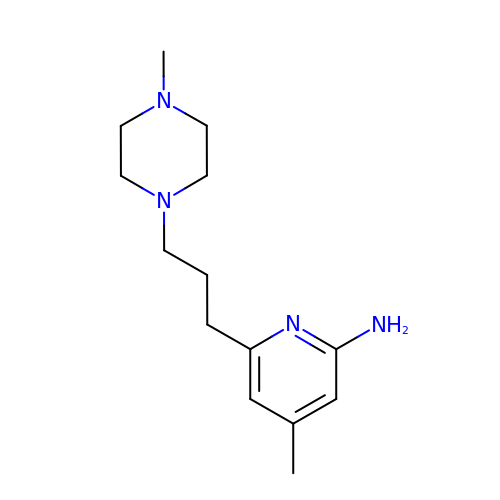4-methyl-6-[3-(4-methylpiperazin-1-yl)propyl]pyridin-2-amine | C14 H24 N4 | SJKIQNSRANOUEL-UHFFFAOYSA-N>QTIQPGTGYNNGYFYSYWNDGHGGVTYTNGPGGQFSVNWSNSGNFVGGKGWQPGTKNKVINFSGSYNPNGNSYLSVYGWSRNPLIEYYIVENFGTYNPSTGATKLGEVTSDGSVYDIYRTQRVNQPSIIGTATFYQYWSVRRNHRSSG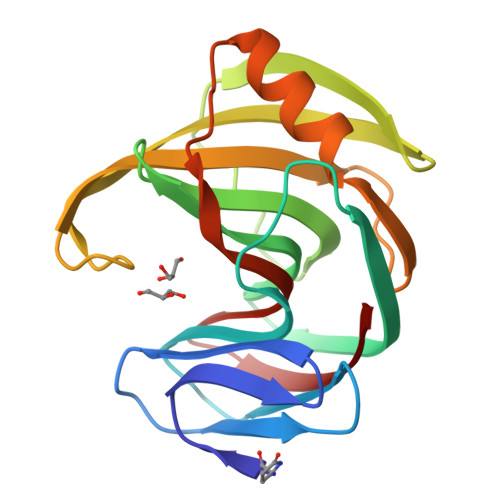SVNTANHFNAWAQQGLTLGTMDYQIVAVEGYFSSGSASITVS[2x]>[6x]MRKIALFPGSFDPMTNGHLNLIERSAKLFDEVIIGVFIN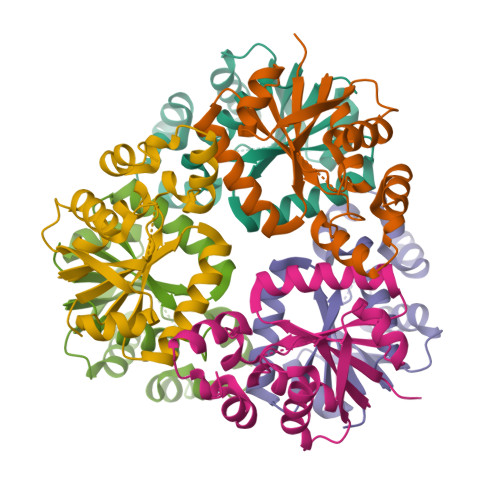TSKQTLFTPEEKKYLIEEATKEMPNVRVIMQETQLTVESAKSLGANFLIRGIRNVKDYEYEKDIAKMNQHLAPEIETVFLLAEEPYAHVSSSLLKEVLRFGGDVSDYLPPNIYHALKQKKNDWSLEHHHHHH>[4x]MGSLVCVGTGLQLAGQISVLSRSYIEHADIVFSLLPDGFSQRWLTKLNPNVINLQQFYAQNGEVKNRRDTYEQMVNAILDAVRAGKKTVCALYGHPGVFACVSHMAITRAKAEGFSAKMEPGISAEACLWADLGIDPGNSGHQSFEASQFM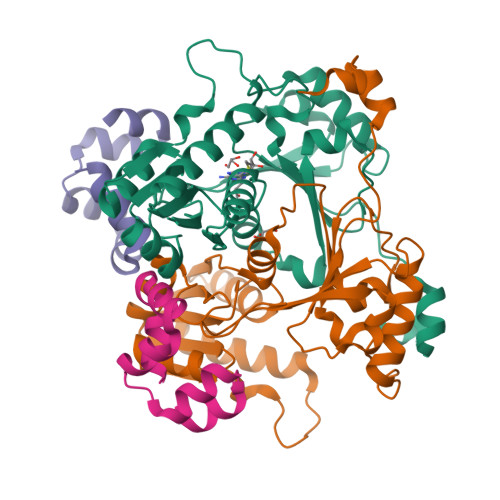FFNHVPDPTTHLLLWQIAIAGEHTLTQFHTSSDRLQILVEQLNQWYPLDHEVVIYEAANLPIQAPRIERLPLANLPQAHLMPISTLLIPPAKKLEYNYAILAKLGIGPEDLG;>MSGLSDFFTQLGQDAQLMEDYKQNPEAVMRAHGLTDEQINAVMTGDMEKLKTLSGDSSYQSYLVISHGNGD[4x]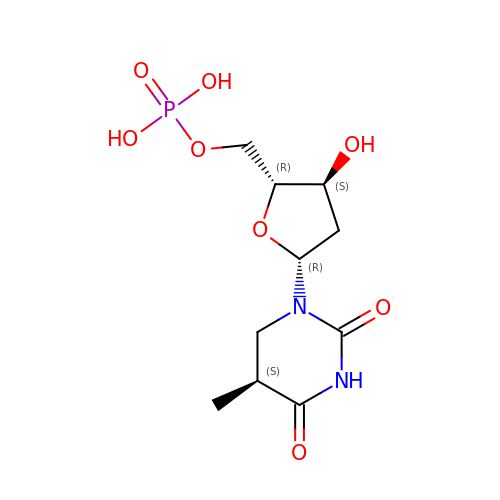[(2R,3S,5R)-3-HYDROXY-5-[(5S)-5-METHYL-2,4-DIOXO-1,3-DIAZINAN-1-YL]OXOLAN-2-YL]METHYL DIHYDROGEN PHOSPHATE | C10 H17 N2 O8 P | PGRQANKWVMVANW-RULNZFCNSA-N>WGKEGHEIICKIAQTRLDETAAKAVKELLPESAEGDLSSLCLWADRVKFRYHWSSPLHYINTPDACSYQYNRDCKDESGEKGRCVAGAIYNYTTQLLSYKTAASSQSQYNLTEALLFVSHFMGDIHQPLHVSYASDKGGNTIEVHWYTRKANLHHIWDSNIIETAEADLYNSALEGMVDALKKNITTEWADQVKRWETCTKKTACPDIYASEGIQAACDWAYKGVTEGDTLE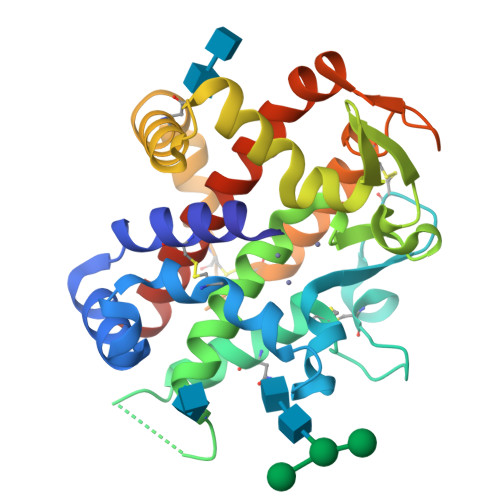DEYFYSRLPIVYQRLAQGGVRLAATLNRIFGHHHHHH[2x]>[4x]MASMTGGNNMGRGSMGAMDQEIGTVTDTKMDPRDFLQL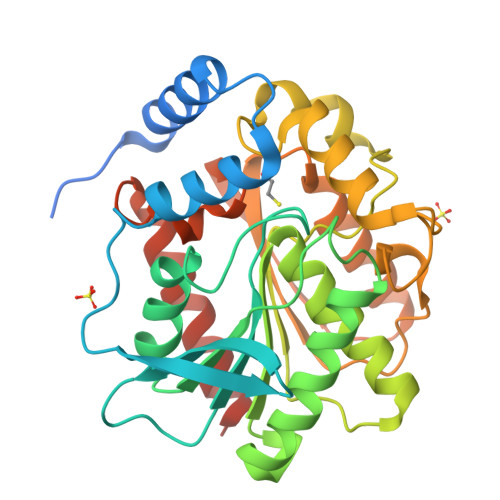LKINAEKAEKNLPLDQKRAGMEALCERFPRAEGVELTLTDLGGVPCIRQATDGAGAAHILYFHGGGYISGSPSTHLVLTTQLAKQSSATLWSLDYRLAPENPFPAAVDDCVAAYRALLKTAGSADRIIIAGDSAGGGLTTASMLKAKEDGLPMPAGLVMLSPFVDLTLSRWSNSNLADRDFLAEPDTLGEMSELYVGGEDRKNPLISPVYADLSGLPEMLIHVGSEEALLSDSTTLAERAGAAGVSVELKIWPDMPHVFQMYGKFVNAADISIKEICHWISARISKLAAALEHHHHHH> MRTPATVVAGVDLGDAVFAAAVRAGVARVEQLMDTELRQADEVMSDSLLHLFNAGGKRFRPLFTVLSAQIGPQPDAAAVTVAGAVIEMIHLATLYHDDVMDEAQVRRGAPSANAQWGNNVAILAGDYLLATASRLVARLGPEAVRIIADTFAQLVTGQMRETRGTSENVDSIEQYLKVVQEKTGSLIGAAGRLGGMFSGATDEQVERLSRLGGVVGTAFQIADDIIDIDSESDESGKLPGTDVREGVHTLPMLYALRESGPDCARLRALLNGPVDDDAEVREALTLLRASPGMARAKDVLAQYAAQARHE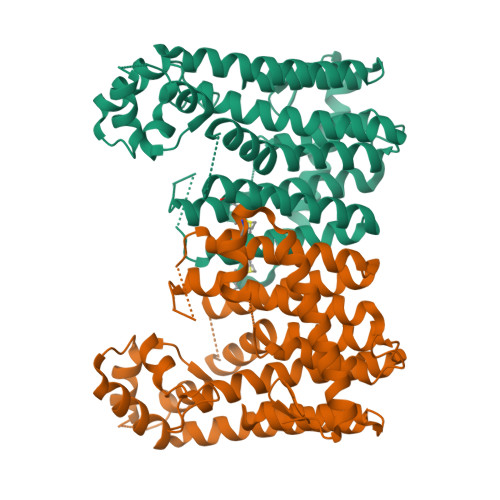LALLPDVPGRRALAALVDYTVSRHG> MPNFSGNWKIIRSENFEELLKVLGVNVMLRKIAVAAASKPAVEIKQEGDTFYIKTSTTVRTTEIN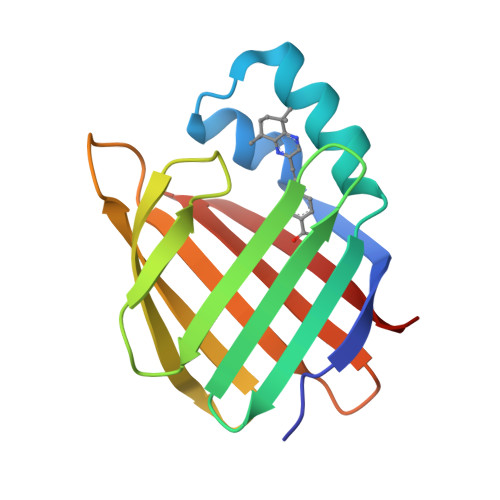FKVGEEFEEQTVDGRPCKSLVKWESENKMVCEQKLLKGEGPKTSWTRELTNDGELILTMTADDVVCTRVYVRE> MSKFLDRFRYFKQKGETFADGHGQLLNTNRDWEDGYRQRWQHDKIVRSTSGVNCTGSCSWKIYVKNGLVTWETQQTDYPRTRPDLPNHEPRGCPRGASYSWYLYSANRLKYPMMRKRLMKMWREAKALHSDPVEAWASIIEDADKAKSFKQARGRGGFVRSSWQEVNELIAASNVYTIKNYGPDRVAGFSPIPAMSMVSYASGARYLSLIGGTCLSFYDWYCDLPPASPQTWGEQTDVPESADWYNSSYIIAWGSNVPQTRTPDAHFFTEVRYKGTKTVAVTPDYAEIAKLCDLWLAPKQGTDAAMALAMGHVMLREFHLDNPSQYFTDYVRRYTDMPMLVMLEERDGYYAAGRMLRAADLVDALG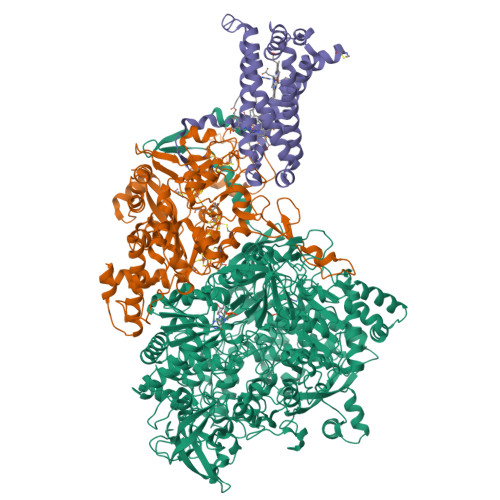QENNPEWKTVAFNTNGEMVAPNGSIGFRWGEKGKWNLEQRDGKTGEETELQLSLLGSQDEIAEVGFPYFGGDGTEHFNKVELENVLLHKLPVKRLQLADGSTALVTTVYDLTLANYGLERGLNDVNCATSYDDVKAYTPAWAEQITGVSRSQIIRIAREFADNADKTHGRSMIIVGAGLNHWYHLDMNYRGLINMLIFCGCVGQSGGGWAHYVGQEKLRPQTGWQPLAFALDWQRPARHMNSTSYFYNHSSQWRYETVTAEELLSPMADKSRYTGHLIDFNVRAERMGWLPSAPQLGTNPLTIAGEAEKAGMNPVDYTVKSLKEGSIRFAAEQPENGKNHPRNLFIWRSNLLGSSGKGHEFMLKYLLGTEHGIQGKDLGQQGGVKPEEVDWQDNGLEGKLDLVVTLDFRLSSTCLYSDIILPTATWYEKDDMNTSDMHPFIHPLSAAVDPAWEAKSDWEIYKAIAKKFSEVCVGHLGKETDIVTLPIQHDSAAELAQPLDVKDWKKGECDLIPGKTAPHIMVVERDYPATYERFTSIGPLMEKIGNGGKGIAWNTQSEMDLLRKLNYTKAEGPAKGQPMLNTAIDAAEMILTLAPETNGQVAVKAWAALSEFTGRDHTHLALNKEDEKIRFRDIQAQPRKIISSPTWSGLEDEHVSYNAGYTNVHELIPWRTLSGRQQLYQDHQWMRDFGESLLVYRPPIDTRSVKEVIGQKSNGNQEKALNFLTPHQKWGIHSTYSDNLLMLTLGRGGPVVWLSEADAKDLGIADNDWIEVFNSNGALTARAVVSQRVPAGMTMMYHAQERIVNLPGSEITQQRGGIHNSVTRITPKPTHMIGGYAHLAYGFNYYGTVGSNRDEFVVVRKMKNIDWLDGEGNDQVQESVK;> MKIRSQVGMVLNLDKCIGCHTCSVTCKNVWTSREGVEYAWFNNVETKPGQGFPTDWENQEKYKGGWIRKINGKLQPRMGNRAMLLGKIFANPHLPGIDDYYEPFDFDYQNLHTAPEGSKSQPIARPRSLITGERMAKIEKGPNWEDDLGGEFDKLAKDKNFDNIQKAMYSQFENTFMMYLPRLCEHCLNPACVATCPSGAIYKREEDGIVLIDQDKCRGWRMCITGCPYKKIYFNWKSGKSEKCIFCYPRIEAGQPTVCSETCVGRIRYLGVLLYDADAIERAASTENEKDLYQRQLDVFLDPNDPKVIEQAIKDGIPLSVIEAAQQSPVYKMAMEWKLALPLHPEYRTLPMVWYVPPLSPIQSAADAGELGSNGILPDVESLRIPVQYLANLLTAGDTKPVLRALKRMLAMRHYKRAETVDGKVDTRALEEVGLTEAQAQEMYRYLAIANYEDRFVVPSSHRELAREAFPEKNGCGFTFGDGCHGSDTKFNLFNSRRIDAIDVTSKTEPHP;> MQFLNMFFFDIYPYIAGAVFLIGSWLRYDYGQYTWRAASSQMLDRKGMNLASNLFHIGILGIFVGHFFGMLTPHWMYEAWLPIEVKQKMAMFAGGASGVLCLIGGVLLLKRRLFSPRVRATTTGADILILSLLVIQCALGLLTIPFSAQHMDGSEMMKLVGWAQSVVTFHGGASQHLDGVAFIFRLHLVLGMTLFLLFPFSRLIHIWSVPVEYLTRKYQLVRARH> GSHMSGIALSRLAQERKAWRKDHPFGFVAVPTKNPDGTMNLMNWECAIPGKKGTPWEGGLFKLRMLFKDDYPSSPPKCKFEPPLFHPQVYPSGTVCLSILEEDKDWRPAITIKQILLGIQELLNEPNIQDPAQAEAYTIYCQNRVEYEKRVRAQAKKFAPS;> STGEPAPVLSSPPPADVSTFLAFPSPEKLLRLGPKSSVLIAQQTDTSDPEKVVSAFLKVSSVFK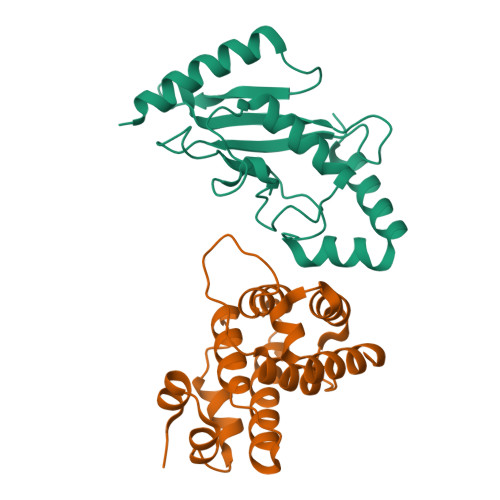DEATVRMAVQDAVDALMQKAFNSSSFNSNTFLTRLLVHMGLLKSEDKVKAIANLYGPLMALNHMVQQDYFPKALAPLLLAFVTKPNSALESCSFARHSLLQTLYKV>LVIMLYVFHRKRNNSRLGNGVLYASVNPEYFSAADVYVPDEWEVAREKITMSRELGQGSFGMVYEGVAKGVVKDEPETRVAIKTVNEAASMRERIEFLNEASVMKEFNCHHVVRLLGVVSQGQPTLVIMELMTRGDLKSYLRSLRPEMENNPVLAPPSLSKMIQMAGEIADGMAYLNANKFVHRDLAARNCMVAEDFTVKIGDFGMTRDIYETDYYRKGGKGLLPVRWMSPESLKDGVFTTYSDVWSFGVVLWEIATLAEQPYQGLSNEQVLRFVMEGGLLDKPDNCPDMLFEL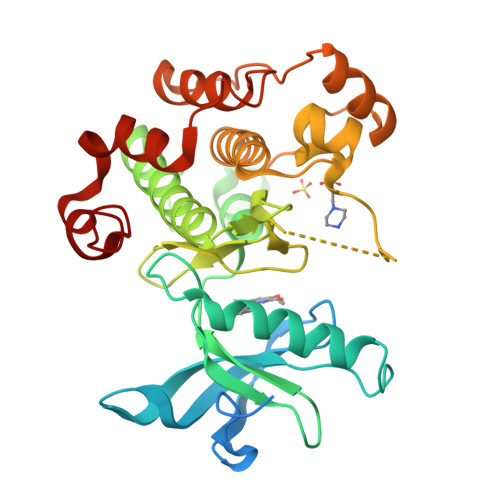MRMCWQYNPKMRPSFLEIISSIKEEMEPGFREVSFYYSEENK[4x]>MGSHHHH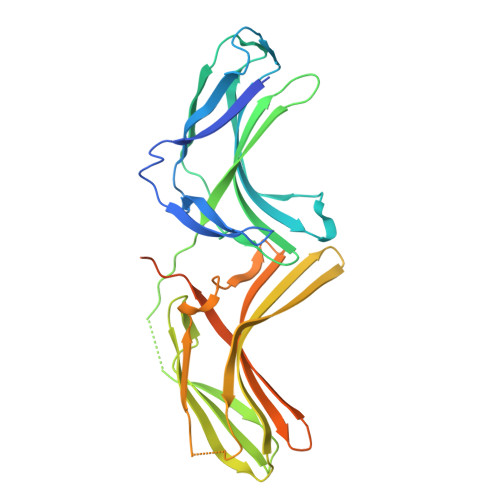HHMGQSVEVEILLNDAESRKRAEHKTEDGKKEKYFLFYDGETVSGKVSLSLKNPNKRLEHQGIKIEFIGQIELYYDRGNHHEFVSLVKDLARPGEITQSQAFDFEFTHVEKPYESYTGQNVKLRYFLRATISRRLNDVVKEMDIVVHTLSTYPELNSSIKMEVGIEDCLHIEFEYNKSKYHLKDVIVGKIYFLSVEIKIKHMEIDIIKRETTGTGPNVYHENDTIAKYEIMDGAPVRGSSIPIRLFLAGYELTPTMRDINKKFSVRYYLNLVLIDEEERRYFKQQEVVLWRKGDIVRKSMSHQAAIASQRFEGTTSLGEVRTPGQLSDNNSRQ[2x]>GPMEQLKCCSGILKEMFAKKHAAYAWPFYKPVDVEALGLHDYCDIIKHPMDMSTIKSKLEAREYRDAQEFGADVRLMF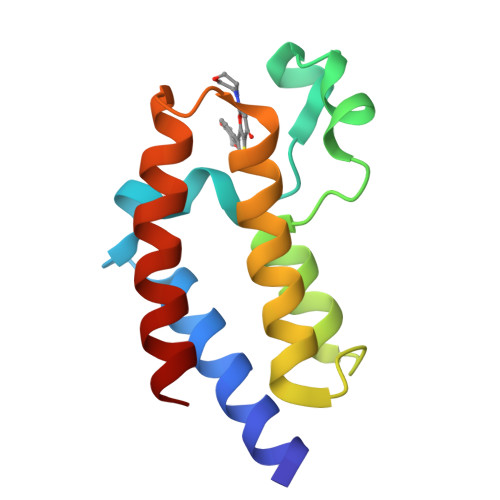SNCYKYNPPDHEVVAMARKLQDVFEMRFAKM[2x]2-[[4-chloranyl-2,6-bis(fluoranyl)phenyl]methylamino]-7-oxidanylidene-5-propyl-4H-pyrazolo[1,5-a]pyrimidine-3-carbonitrile | C17 H14 Cl F2 N5 O | 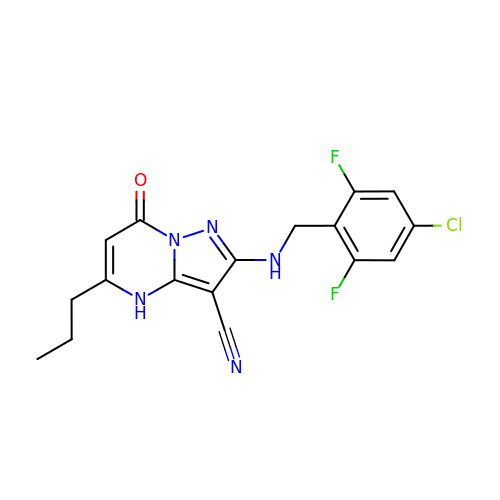SFUVDTPAOHEGCQ-UHFFFAOYSA-N> LY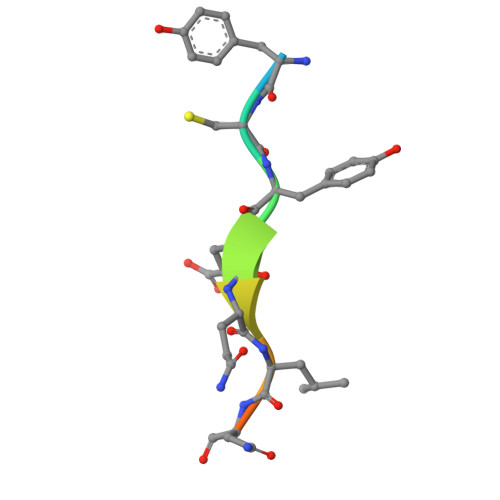CYEQLNDEE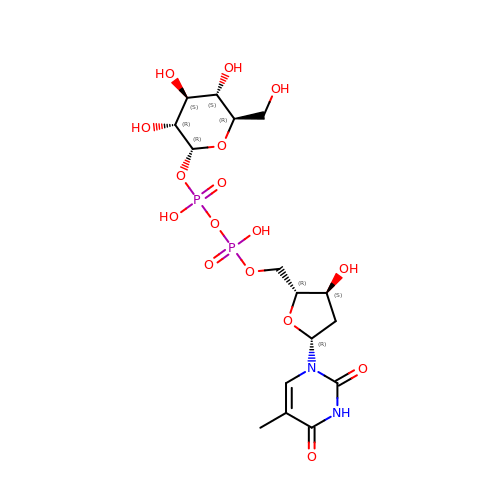2'DEOXY-THYMIDINE-5'-DIPHOSPHO-ALPHA-D-GLUCOSE | C16 H26 N2 O16 P2 | YSYKRGRSMLTJNL-URARBOGNSA-N> GPMPGKSVV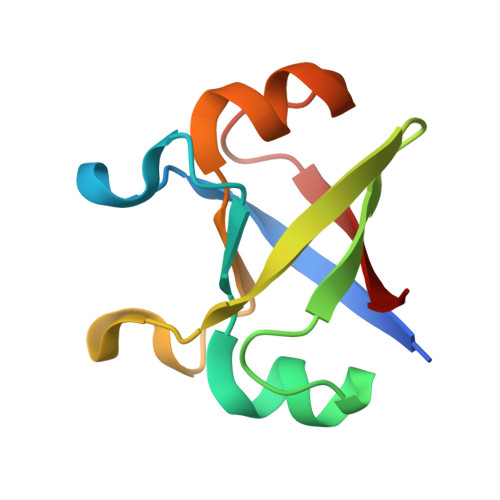ARVAEAYPEDVGKRIVRMDKYERAKLGVSVGDYVEVKKVKSVVARVAEAYPEDVGKRIVRMDKYERAKLGVSVGDYVEVKKV> MLWQKPTAPEQAPAPARPYQGVRVKEPVKELLRRKRGHASSGA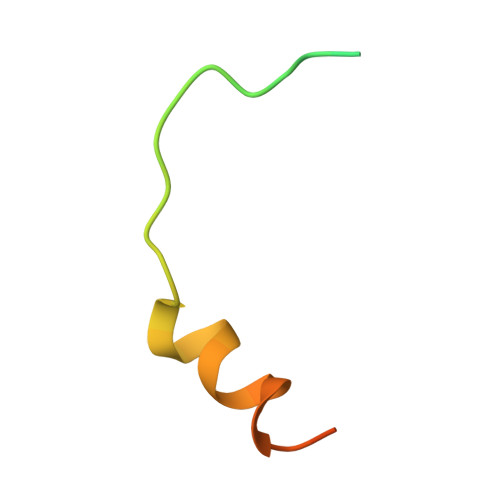A> MTTITYDTDLLPPPELKVPSLDQALAPESVKNDDPFLDLSYFPVPKGFDNVGSLELNNLS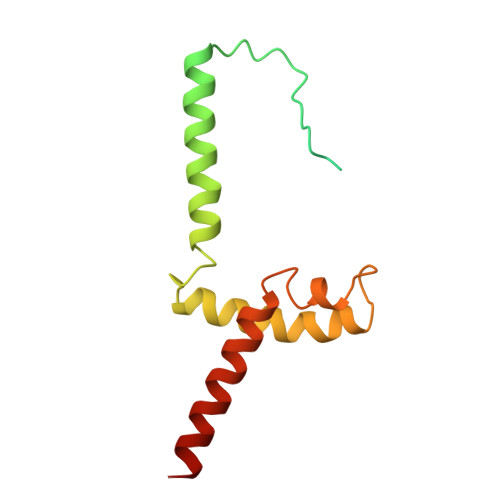TAEDVATLQNQLNKLAEEKHKRSTWKGLTFRIAVQDMWEALTGIPTDIYQNSGRVSLKELLTRDDRLRGLGLIFFLVAVVSIFFLAAG>[2x]MNPILRNPMEAMYPHIFYFHFKNLRKAYGRNESWLCFTMEVVKHHSPVSWKRGVFRNQVDPETHCHAERCFLSWFCDDILSPNTNYEVTWYTSWSPCP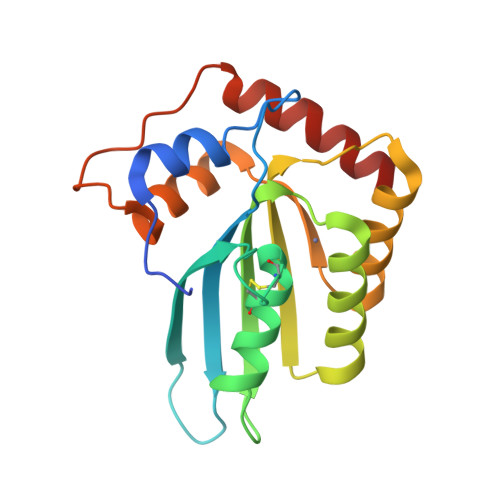ECAGEVAEFLARHSNVNLTIFTARLYYFWDTDYQEGLRSLSQEGASVEIMGYKDFKYCWENFVYNDDEPFKPWKGLKYNFLFLDSKLQEILE> GPLGSMENSCNFNNSIKNVIVFYINEKALIEEKKMLSCYENKLLNLIKEDCENIMLKYKPNLSYICSLLKVDDTSEENIKHIKDQIIESLENDNRPSVKLAIISLISMIVEM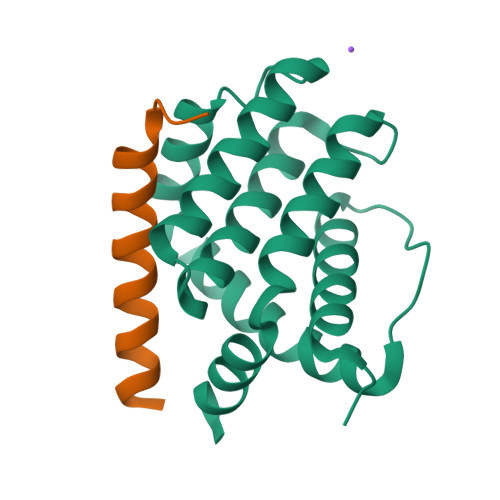NGYKGKNIPMSFLIEDIALKISENSEDLINFINIKNKQKS;> EEQWAREIGAQLRRMADDLNAQYERR> RLYWDDLKRKLSEKLDSTDFTSTIKLLNENSYVPREAGSQKDENLALYVENQFREFKLSKVWRDQHFVKIQVKDSAQNSVIIVDKNGRLVYLVENPGGYVAYSKAATVTGKLVHANFGTKKDFEDLYTPVNGSIVIVRAGKITFAEKVANAESLNAIGVLIYMDQTKFPIVNAELSFFGHAHLGTGDPYTPGFPSFNHTQFPPSRSSGLPNIPVQTISRAAAEKLFGNMEGDCPSDWKTDSTCRMVTSESKNVKLTVSNVLKEIKILNIFGVIKGFVEPDHYVVVGAQRDAWGPGAAKSGVGTALLLKLAQMFSDMVLKDGFQPSRSIIFASWSAGDFGSVGATEWLEGYLSSLHLKAFTYINLDKAVLGTSNFKVSASPLLYTLIEKTMQNVKHPVTGQFLYQDSNWASKVEKLTLDNAAFPFLAYSGIPAVSFCFCEDTDYPYLGTTMDTYKELIERIPELNKVARAAAEVAGQFVIKLTHDVELNLDYERYNSQLLSFVRDLNQYRADIKEMGLSLQWLYSARGDFFRATSRLTTDFGNAEKTDRFVMKKLNDRVMRVEYHFLSPYVSPKESPFRHVFWGSGSHTLPALLENLKLRKQNNGAFNETLFRNQLALATWTIQGAANALSGDVWDIDNEF;> NHSNELPSLCMLNNSFYYMRGGVNTFLIRVSDISVLMKEYDVSIYEPEDLGNCLNKSDSS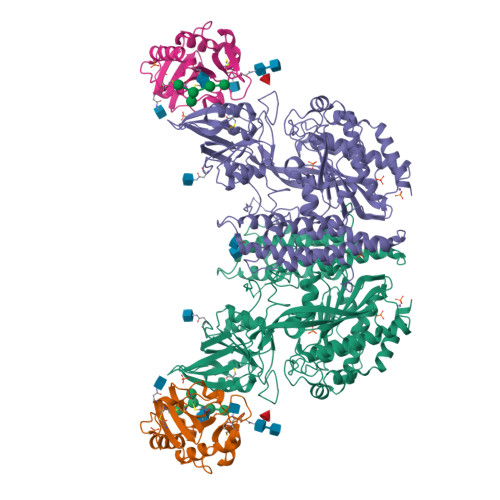WAIHWFSNALGHDWLMDPPMLCRNKTKKEGSNIQFNISKADDARVYGKKIRNGMRHLFRGFHDPCEEGKVCYLTINQCGDPSSFDYCGVNHLSKCQFDHVNT> GHMKQQQTVILYPSPGVGHIVPMVQLAKVFLRHGCDVTMVIAEPAASSPDFRIVDLDRVAASNPAITFHVLPPVPYADLAVPGKHHFLLTLQVLRRYNGE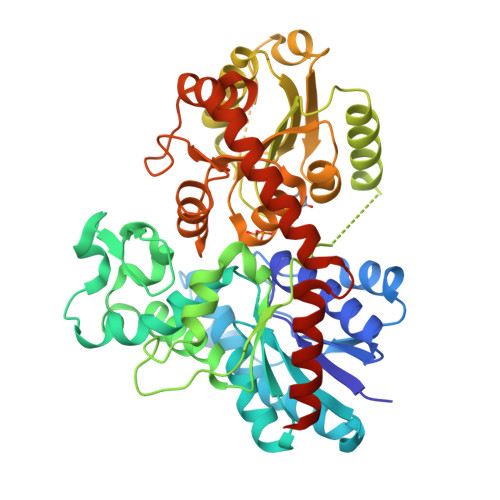LERFLRSVPRERLHSLVVGMFCTDAVDVGAKLGVPVYTFFASAAATLAVVAQLPALLSGRRAGLKELGDTPLQFLGVPPFPASHLVRELLEHPDDDELCKTMVDVWKRCTDGSGVLVNTFESLESPAVQALRDPRCVPGRVLPPVYCVGPLIGGDGGTRAAAEQERAAETRHECLAWLDEQPENSVVFLCFGSRCAHSAEQLRGIAVGLERSGQRFLWSVRTPAGTDGGSENLGALFPEGFLQRTKDRGLVVRSWAPQVEVLRHPSTGAFMTHCGWNSTLEAITAGVPMLCWPFYAEQLMNKVFVTEGMGVGVEMEGYTTGFIKSEEVEAKVRLVMESEEGRHLRGRAVALKNEAQAALRDDGPSETSFARFLFDAKNLQGHLGHGSE>AAAASAPPAPADALPKGADSFFRTVISNMEKVYLSRNPTAKTILELVRSYDGDHICYDHFAFRTFGVDGYGIKSLAEFFTDFGYVPREELRFPAKKLRALWFSPPTNDGYTGTGVYGPLPRIFISELLVDELSPQSQDIIQKYIRTSGKGNKHATLASTSGELTWEKPIYSDFQVLSRESEYAAWTLVNGYALNHTTISTHRLISDIRSINKFNKFVEDNGFKLNSEGGILKVSPDGLLQQSSTVADSALFTFADGITESIPRSYIEFAERLVLPQFKDLPNDEVNEHHRRDGFEVGNADKIFESTSNDQLTRRSAHHHHHH[4x]

In this step, 2OA is converted to D-2-hydroxyglutarate (2HG) in a reaction catalyzed by the Fe(II)-dependent DUF1338 family enzyme hydroxyglutarate synthase (HglS). Homologs of this enzyme are broadly distributed across multiple domains of life, including nearly every sequenced plant genome. Conversion of 2OA directly to D-2HG requires two discrete chemical steps, a decarboxylation and hydroxylation, making the chemical mechanism of the enzyme puzzling. We further show that despite very low sequence identity, plant homologs also catalyze the conversion of 2OA to 2HG and adopt the same structural fold as the bacterial enzyme, suggesting that DUF1338 family proteins catalyze the last unknown step of plant lysine catabolism.

Soluble variants of plant proteins were constructed by removing the predicted N-terminal localization peptide. As expected, the E. coli homolog YdcJ and the plant homologs AT1G07040 and FLO7 catalyzed the conversion of 2OA to that was confirmed by in vitro assays analyzed using high resolution LC-MS. In addition, the FLO7 homolog displayed kinetic parameters similar to HglS, with a Km of 0.55 mM and a Vmax of 0.89 mM/min/µM enzyme. In addition, the structural conservation between bacterial and eukaryotic DUF1338 proteins was compared by obtaining a crystal structure of FLO7. Initial crystallization screens resulted in crystals that were soaked with 2OA, producing diffraction data used to solve the substrate-bound crystal structure at 1.85 Å resolution. The FLO7 crystal structure, like the other DUF1338 proteins, displayed the conserved central VOC fold containing the active site and metal-binding center. Comparison of the HglS and FLO7 structures revealed that orientation of the metal-coordinating residues and 2OA in both structures were nearly identical even though the proteins display low (~15%) sequence identity. In addition, the FLO7 structure also contains a substrate-binding arginine, Arg64, located in nearly the same position as Arg74 of HglS. However, unlike Val402 and Ser403 of HglS, FLO7 does not possess any other residues interacting with the substrate. The results of our biochemical and structural studies of FLO7 manifest the remarkable conservation of the fold, active site architecture, and mechanism among DUF1338 proteins across different domains of life.>[4x]WSHPQFEKVPIKYLPEENVHDADFGEQKDISEINLAAGLDLFQGDILLQKSRNGLRDPNTRWTFPIPYILADNLGLNAKGAILYAFEMFRLKSCVDFKPYEGESSYIIFQQFDGCWSEVGDQHVGQNISIGQGCAYKAIIEHEILHALGFY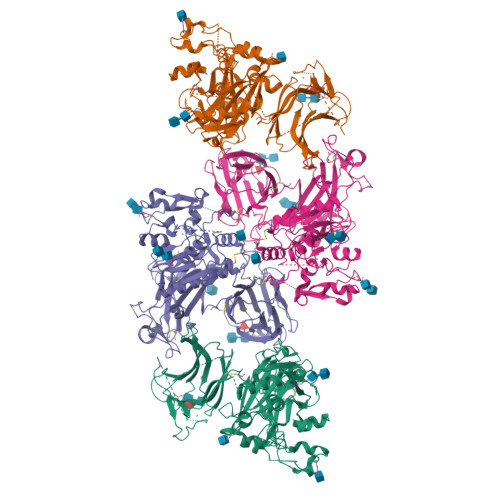HEQSRTDRDDYVNIWWDQILSGYQHNFDTYDDSLITDLNTPYDYESLMHYQPFSFNKNASVPTITAKIPEFNSIIGQRLDFSAIDLERLNRMYNCTTTHTLLDHCTFEKANICGMIQGTRDDTDWAHQDSAQAGEVDHTLLGQCTGAGYFMQFSTSSGSAEEAALLESRILYPKRKQQCLQFFYKMTGSPSDRLVVWVRRDDSTGNVRKLVKVQTFQGDDDHNWKIAHVVLKEEQKFRYLFQGTKGDPQNSTGGIYLDDITLTETPCPTGVWTVRNFSQVLENTSKGDKLQSPRFYNSEGYGFGVTLYPNSRESSGYLRLAFHVCSGENDAILEWPVENRQVIITILDQEPDVRNRMSSSMVFTTSKSHTSPAINDTVIWDRPSRVGTYHTDCNCFRSIDLGWSGFISHQMLKRRSFLKNDDLIIFVDFEDITHLS> EGSITQGTPLKY;> FTTGLVYDTLMLKHQCTCGSSSSHPEHAGRIQSIWSRLQETGLRGKCECIRGRKATLEELQTVHSEAHTLLYGTNPLNRQKLDSKKLLGSLASVFVRLPCGGVGVDSDTIWNEVHSAGAARLAVGCVVELVFKVATGELKNGFAVVRPPGHHAEESTPMGFCYFNSVAVAAKLLQQRLSVSKILIVDWDVHHGNGTQQAFYSDPSVLYMSLHRYDDGNFFPGSGAPDEVGTGPGVGFNVNMAFTGGLDPPMGDAEYLAAFRTVVMPIASEFAPDVVLVSSGFDAVEGHPTPLGGYNLSARCFGYLTKQLMGLAGGRIVLALEGGYDLTAICDASEACVSALLGNELDPLPEKVLQQRPNANAVRSMEKVMEIHSKYWRCLQRTTSTAGRSLIEAQTCEN

The HDAC domains of class IIa HDACs repress the respective target genes by interacting with the C-terminal region of the silencing mediator for retinoid and thyroid receptor (SMRT) repression domain 3 (SRD3c). Here, we found that two conserved GSI-containing motifs of SRD3c are critical for HDAC4 binding. Two SMRT peptides including these motifs commonly form a β-hairpin structure in the cleft and block the catalytic entry site of HDAC4. They interact mainly with class IIa HDAC-specific residues of HDAC4 in a closed conformation.

For the SRD3c protein, we designed two peptides (SP1: −3HIRGSITQGIPRSYV+12, SP2: −2KEGSITQGTPLKY+11), which include the GSI motif in the sequences. For kinetic analysis of peptide binding to HDAC4c H976Y (R651-T1055), we performed ITC experiments and obtained a dissociation constant of 2.23 μM for SP1 and 18.8 μM for SP2. Consistent with this, these peptides inhibited the in vitro deacetylase activity of HDAC4c H976Y, with a better inhibitory effect of SP1 than that of SP2. Overall, the refined HDAC4c-peptide structures superpose well on the apo-form structure, indicating that peptides binding did not rearrange the catalytic and structural zinc ion-binding sites. The bound peptides commonly form a β-hairpin structure of two β-strands in the HDAC4c cleft leading to the catalytic zinc ion. The hydrophobic I+3 residues (I1363 or I1459) are at the β-turn near the catalytic zinc ion and intervened with F812 and F871 at the end of the cleft and entrance to the catalytic pocket of the HDAC4c. At one side of the cleft, a water molecule (w4) mediates the interaction between the carbonyl oxygen of I+3 in both peptides with the side-chain of H842 of the catalytic subdomain. At the two loops of S744–W762 and H803–G811 of the structural zinc ion-binding site, D759 hydrogen-bonds with the hydroxyl group of T+4 and peptidyl nitrogen atom between S+2 and I+3 in two peptides. Notably, D757 interacts indirectly with R+9 of the bound SP1 via a water molecule (w8), which is missing in the SP2-bound structure with L+9 at the corresponding position. The two motifs are very close to each other, with a major difference in the structurally relevant positions R+9 in SM1 and L+9 in SM2.>[8x]MTSVTSKQSTILGSDEIDLGRVIGELIDHRKLIISITSVFTLFAILYALLATPIYETDALIQIEQKQGNAILSSLSQVLPDGQPQSAPETALLQSRMILGKTIDDLNLQIQIEQKYFPVIGRGLARLMGEKPGNIDITRLYLPDSDDISNNTPSIILTVKDKEN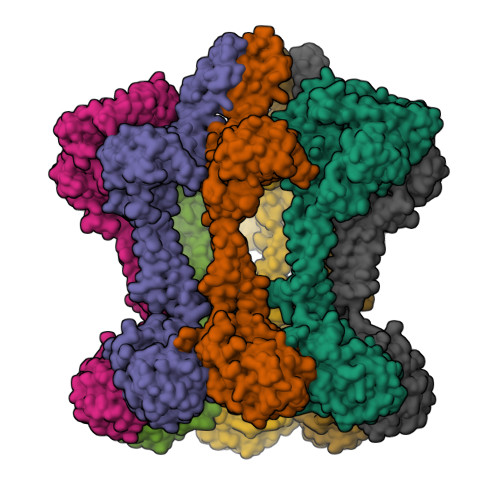YSINSDGIQLNGVVGTLLNEKGISLLVNEIDAKPGDQFVITQLPRLKAISDLLKSFSVADLGKDTGMLTLTLTGDNPKRISHILDSISQNYLAQNIARQAAQDAKSLEFLNQQLPKVRAELDSAEDKLNAYRKQKDSVDLNMEAKSVLDQIVNVDNQLNELTFREAEVSQLYTKEHPTYKALMEKRQTLQEEKSKLNKRVSSMPSTQQEVLRLSRDVESGRAVYLQLLNRQQELNIAKSSAIGNVRIIDNAVTDPNPVRPKKTIIIVIGVVLGLIVSVVLVLFQVFLRRGIESPEQLEEIGINVYASIPISEWLTKNARQSGKVRKNQSDTLLAVGNPADLAVEAIRGLRTSLHFAMMEAKNNVLMISGASPSAGMTFISSNLAATIAITGKKVLFIDADLRKGYAHKMFGHKNDKGLSEFLSGQAAAEMIIDKVEGGGFDYIGRGQIPPNPAELLMHPRFEQLLNWASQNYDLIIIDTPPILAVTDAAIIGRYAGTCLLVARFEKNTVKEIDVSMKRFEQSGVVVKGCILNGVVKKASSYYRYGHNHEGESEEDKKHHHHHH>[4x]XADEIAKAQVARPGGDTIFGKIIRKEIPAKIIFEDDRCLAFHDISPQAPTHFLVIPKKHISQISVAEDDDESLLGHLMIVGKKCAADL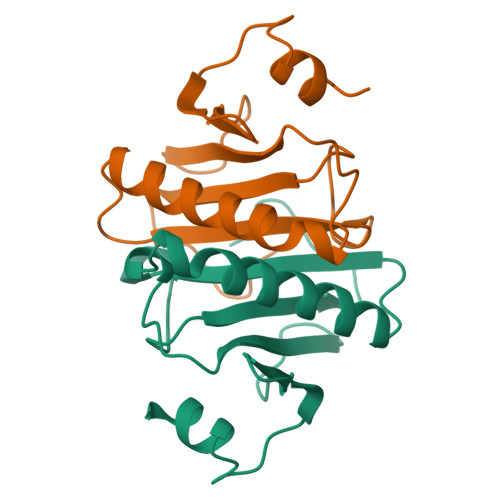GLNKGYRMVVNEGSDGGQSVYHVHLHVLGGRQMHWPPG> MKSVMTTTISAADAAGRFPSSSDLESVQG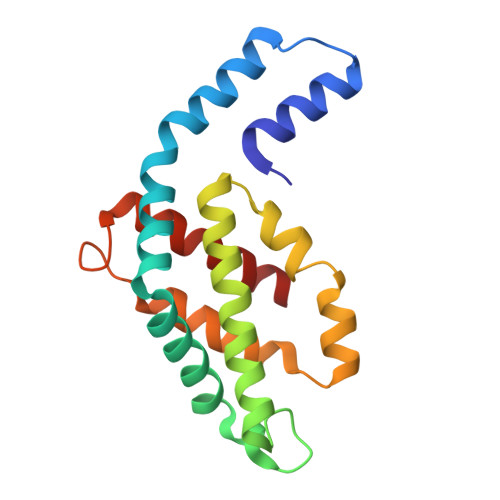NIQRAAARLEAAEKLASNHEAVVKEGGDACFAKYSYLKNPGEAGDSQEKVNKCYRDVDHYMRLVNYSLVVGGTGPLDEWAIAGAREVYRTLNLPSASYVAAFAFTRDRLCVPRDMSAQAGGEYVAALDYIVNALT2,3-dimethoxy-5-[(1S)-1-phenylpropyl]benzene-1,4-diol | C17 H20 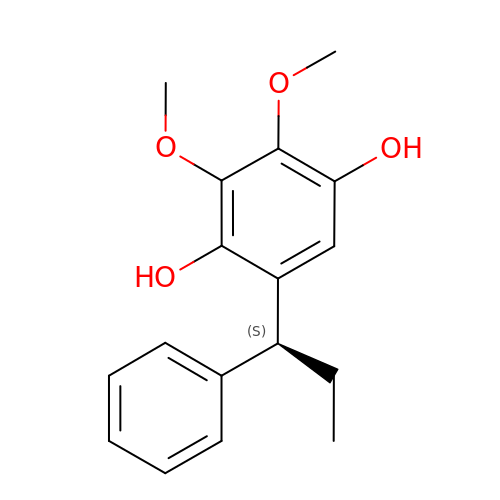O4 | PIKYYJHZIWYFFE-LBPRGKRZSA-N> HHAADYVLYKDATKPVEDR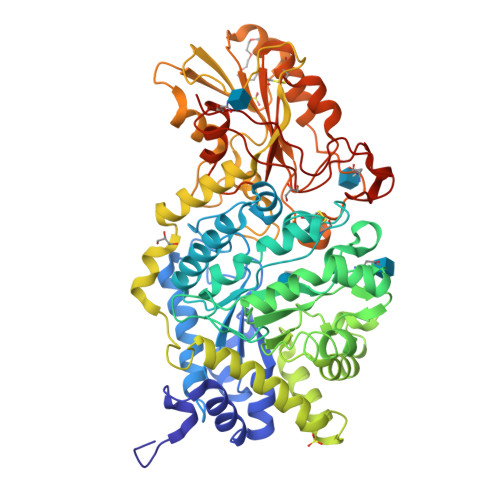VADLLGRMTLAEKIGQMTQIERLVATPDVLRDNFIGSLLSGGGSVPRKGATAKEWQDMVDGFQKACMSTRLGIPMIYGIDAVHGQNNVYGATIFPHNVGLGATRDPYLVKRIGEATALEVRATGIQYAFAPCIAVCRDPRWGRCYESYSEDRRIVQSMTELIPGLQGDVPKDFTSGMPFVAGKNKVAACAKHFVGDGGTVDGINENNTIINREGLMNIHMPAYKNAMDKGVSTVMISYSSWNGVKMHANQDLVTGYLKDTLKFKGFVISDFEGIDRITTPAGSDYSYSVKASILAGLDMIMVPNKYQQFISILTGHVNGGVIPMSRIDDAVTRILRVKFTMGLFENPYADPAMAEQLGKQEHRDLAREAARKSLVLLKNGKTSTDAPLLPLPKKAPKILVAGSHADNLGYQCGGWTIEWQGDTGRTTVGTTILEAVKAAVDPSTVVVFAENPDAEFVKSGGFSYAIVAVGEHPYTETKGDNLNLTIPEPGLSTVQAVCGGVRCATVLISGRPVVVQPLLAASDALVAAWLPGSEGQGVTDALFGDFGFTGRLPRTWFKSVDQLPMNVGDAHYDPLFRLGYGLTTNATKKY Found within a gene class designated "pathogenicity, virulence and adaptation" in the annotated genome of Xanthomonas citri subsp. citri strain 306 is the sodM (XAC2386) gene, which encodes a predicted superoxide dismutase (XcSOD). Superoxide dismutases are metalo-oxidoreductases (EC: 1.15.1.1) that catalyze the dismutation of the superoxide radical (O2•-) into molecular oxygen and hydrogen peroxide (H2O2). Depending on the redox metal cofactor, SODs can be classified into three main structural groups: Cu,ZnSODs which contain both metals, MnSOD/FeSODs which have either one or the other metal, and the NiSODs. Heterologous expression of sodM provided pure, homogeneous, catalytically active XcSOD, from which a high resolution structure was determined by X-ray crystallography.

XcSOD crystallized in space group P212121 with two monomers per asymmetric unit. XcSOD shows the well-known fold characteristic of both MnSOD/FeSODs and presents an overall RMSD of 0.35 Å on Cα atoms when a monomer is superposed on its closest homologue, the MnSOD from B. subtilis, which was used for molecular replacement. In the case of XcSOD the two monomers in the asymmetric unit are related to one another in such a way as to present all of the hallmarks of a dimeric enzyme consistent with the SEC results and the crystallographic symmetry. These are most notably characterised by the lack of the large antiparallel α-helical hairpin composed of α1 and α3 which is typical of tetrameric enzymes. Further analysis of the amino acid sequence also reveals that XcSOD has all of the residues previously identified to be fingerprints of a Mn-containing enzyme and therefore was refined as such. The Mn ion is coordinated by Asp164, His81, His27, His168 and a solvent derived ligand (HOH304). Residues which are important for defining the topography and electrostatic potential of the access channel to the metal are highly conserved and include Trp130 and Trp166 as well as His31,Tyr35 and Gln149 which participate in the conserved network of hydrogen bonds necessary for securing the metal-bound solvent ligand or superoxide. The electrostatic potential around the active site is very similar to that observed in other members of the FeSOD/MnSOD family and presents a halo of positive charge directing the substrate anion towards the active site. With respect to catalysis, XcSOD presented a specific activity of 11609 U/mg, very similar to the value of 12800 U/mg reported for Yersinia enterocolitica SodA, a tetrameric MnSOD with which it shares 57% sequence identity.

>[2x]MAYTLPQLPYAYDALEPNIDAQTMEIHHTKHHQTYINNVNAALEGTEYADLPIEELVSKLKSLPENLQGPVRNNGGGHANHSLFWTVLSPNGGGEPKGEVAKAIDKDLGGFEKFKEAFTKAAVSRFGSGWAWLSVTPDKKLVVESTANQDSPLFEGNTPILGLDVWEHAYYLKYQNRRPEYIGAFYNAVNWEEVERRYHAAIA> VQAVAVLKGDAGVSGVVKFEQASESEPTTVSYEIAGNSPNAERGFHI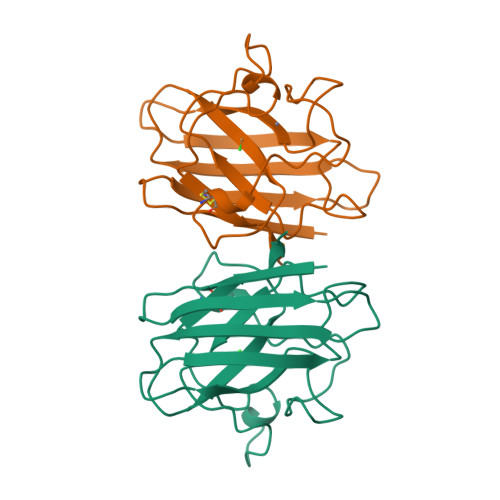CEFGDATNGCVSAGPHFNPFKKTHGAPTDEVRHVGDMGNVKTDENGVAKGSFKDSLIKLIGPTSVVGRSVVIHAGQDDLGKGDTEESLKTGNAGPRPACGVIGLTN>GDTHEFHKLLIKVVDLFLEDRIKEFEMKLNTTLDELEFEELIGKPDSSNSAENNGIFIDEYSYDASENAMKKLFVEYVRQPEFKYTVL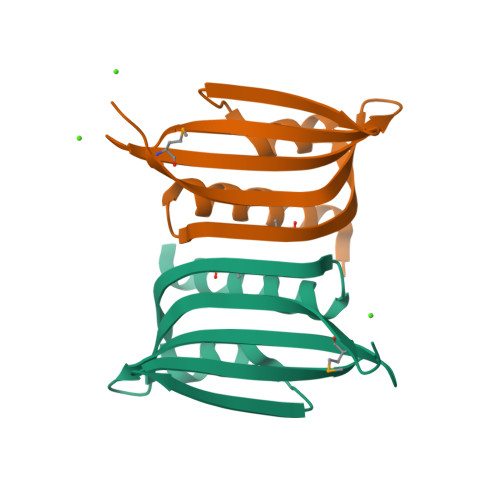SIKGVNDWVRE[4x]>[8x]VKLAGNSSLCPINGWAVYSKDNSIRIGSKGDVFVIREPFISCSHLECRTFFL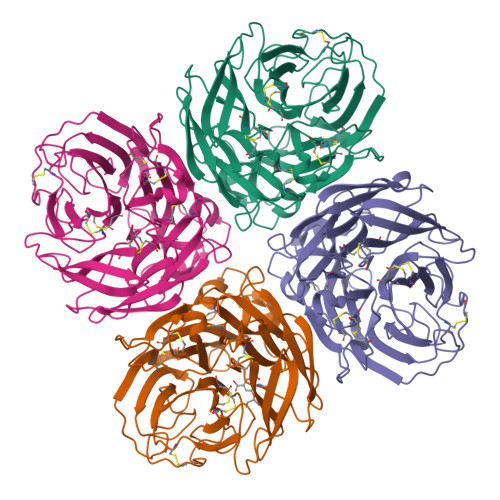TQGALLNDKHSNGTVKDRSPHRTLMSCPVGEAPSPYNSRFESVAWSASACHDGTSWLTIGISGPDNGAVAVLKYNGIITDTIKSWRNNILRTQESECACVNGSCFTVMTDGPSNGQASYKIFKMEKGKVVKSVELDAPNYHYEECSCYPNAGEITCVCRDNWHGSNRPWVSFNQNLEYQIGYICSGVFGDNPRPNDGTGSCGPVSSNGAYGVKGFSFKYGNGVWIGRTKSTNSRSGFEMIWDPNGWTETDSSFSVKQDIVAITDWSGYSGSFVQHPELTGLDCIRPCFWVELIRGRPKESTIWTSGSSISFCGVNSDTVGWSWPDGAELPFTIDK>ADGIQEAKPSGSVVEQAEGVECDFSPLLSGTPPQVYNFKRLVFTNCNYNLTKLLSLFSVNDFTCSQISPAAIASNCY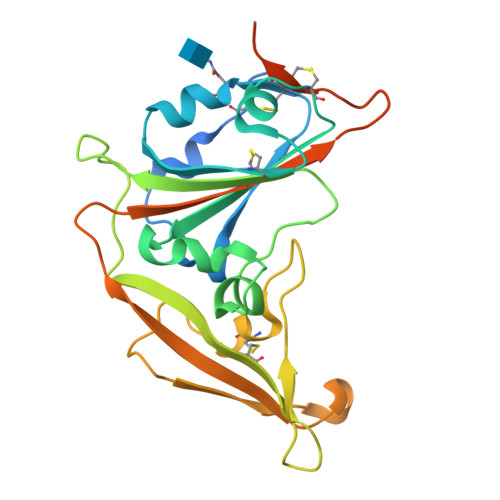SSLILDYFSYPLSMKSDLSVSSAGPISQFNYKQSFSNPTCLILATVPHNLTTITKPLKYSYINKCSRLLSDDRTEVPQLVNANQYSPCVSIVPSTVWEDGDYYRKQLSPLEGGGWLVASGSTVAMTEQLQMGFGITVQYGTDTNSVCPKLEFANDTKIASQLGNCVEYHHHHHH[2x]3-(4-NITRO-PHENOXY)-PROPAN-1-OL 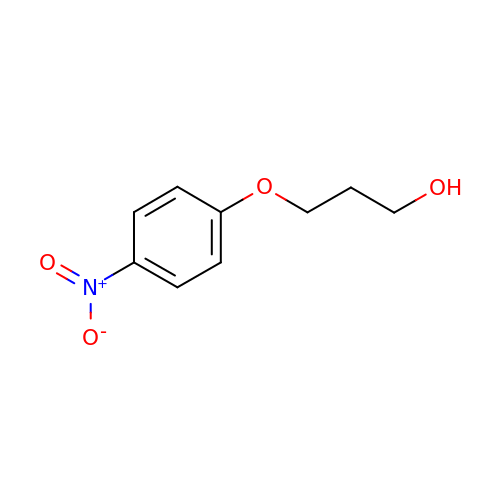| C9 H11 N O4 | XHRNQMMJGWBTBU-UHFFFAOYSA-N Compared to the RdRPs of other Flaviviridae representatives such as the NS5 of the Japanese encephalitis virus (JEV) and dengue virus (DENV) in the Flavivirus genus and the NS5B of the hepatitis C virus (HCV) of the Hepacivirus genus, the pestivirus NS5B contains a unique ∼90-residue N-terminal domain (NTD) that does not have notable sequence homology to any other viral or host proteins. The global conformation of our CSFV NS5B structures is consistent with the recently reported CSFV structure with an RMSD value of 0.9 Å (95% coverage) between the reported structure and our representative C-682 structure. These structures together reveal that the NTD adopts a globular α/β fold with an α-β-α-β-β-α pattern. The NTD interacts with the palm of the RdRP core intra-molecularly with a mixture of hydrophobic and hydrogen bonding interactions. Collectively, these biochemical data indicated that the RNA synthesis fidelity of CSFV NS5B is fine-tuned by its NTD through the intra-molecular interactions with the RdRP palm.

To better understand the nature of the NTD–RdRP intra-molecular interface interactions and whether they regulate the RdRP fidelity, we designed point mutations at the Y471 and E472 sites in the context of the WT NS5B and the N- and C-terminal deletion mutants. Among these five structures, three of them (Y471A and two forms of C-672_Y471A) maintain the WT conformation with the NTD–RdRP intra-molecular interface maintained. The NTD–RdRP intra-molecular interactions are fully disrupted, and the NTD is rather involved in a non-intensive three-way interaction involving two symmetry-related neighboring NS5B molecules in the crystal lattice. These structural data together suggest that the selection of Y471-E472 mutation sites is valid in perturbing the NTD–RdRP interface, but the interface may not necessarily be fully disrupted by some of the mutations. 60-min and 180-min were chosen as representative time points for a comparison also including single-point alanine mutants (Y471A, E472A, and the N-91 form mutants). Consistent with the observation in the time course experiments, every mutant either lacking the NTD or bearing mutation(s) at residues Y471 and E472 showed much higher level of misincorporation than the WT did. The effect of E472A mutation was highly consistent with AA mutation (compare lanes 4/8/14/18 to 5/9/15/19), while the effect of Y471A mutation was slightly smaller than that of the E472A and AA mutations (compare lanes 3/7/13/17 to 4/8/14/18 and 5/9/15/19). Although NTD–RdRP disengagement, a situation mimicked by the crystallographic open conformation state in a crystal lattice or the N-91 construct in solution, results in fidelity reduction, engaged NTD–RdRP with perturbation from point mutations can achieve similar level of fidelity reduction.

> MSNWVMQEENKQGNLTPLFEELLQQCPPGGQNKTAHMVSAYQLAQGNWMPTSCHVFMGTISARRTKTHPYEAYVKLRELVEEHKMKTLCPGSSLGKHNDWIIGKIKYQGNLRTKHMLNPGKVAEQLCREGHRHNVYNKTIGSVMTATGIRLEKLPVVRAQTDTTNFHQAIRDKIDKEENLQTPGLHKKLMEVFNALKRPELESSYDAVEWEELERGINRKGAAGFFERKNIGEILDSEKNKVEEIIDNLKKGRNIKYYETAIPKNEKRDVNDDWTAGDFVDEKKPRVIQYPEAKTRLAITKVMYKWVKQKPVVIPGYEGKTPLFQIFDKVKKEWDQFQNPVAVSFDTKAWDTQVTTKDLELIKDIQKYYFKKKWHKFIDTLTMHMTEVPVICADGEVYIRKGQRGSGQPDTSAGNSMLNVLTMVYAFCEATGVPYKSFDRVAKIHVCGDDGFLITERALGEKFASKGVQILAEAGKPQKITEGDKMKVAYQFDDIEFCSHTPIQVRWSDNTSSYMPGRNTTTILAKMATRLDSSGERGTIAYEKAVAFSFLLMYSWNPLIRRICLLVLSTELQVKPGKSTTYYYEGDPISAYKEVIGHNLFDLKRTSFEKLAKLNLSMSVLGAWTRHTSKRLLQDCVNMGVKEGNWLVNADRLVSSKTGNRYIPGEGHTLQGRHYEELVLARKQINNFQGADRYNGSSSHHHHHH[3-(4-{3-[3-NITRO-5-(GALACTOPYRANOSYLOXY)-BENZOYLAMINO]-PROPYL}-PIPERAZIN-1-YL)-PROPYLAMINO] -2-(3-{4-[3-(3-NITRO-5-[GALACTOPYRANOSYLOXY]-BENZOYLAMINO)-PROPYL]-PIPERAZIN-1-YL} 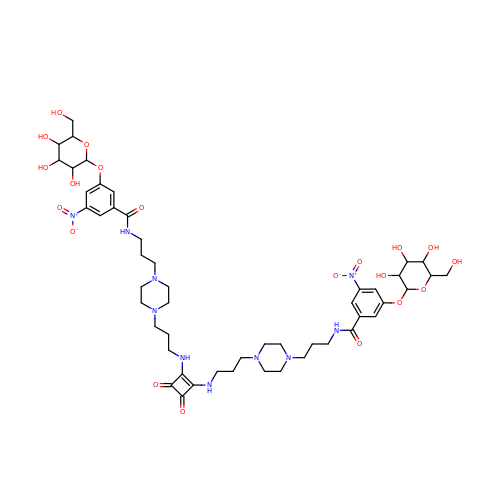-PROPYL-AMINO)-3,4-DIOXO-CYCLOBUTENE | C50 H72 N10 O20 | WWGXKLSKKKQRMN-MLHPNDMTSA-N> GKIND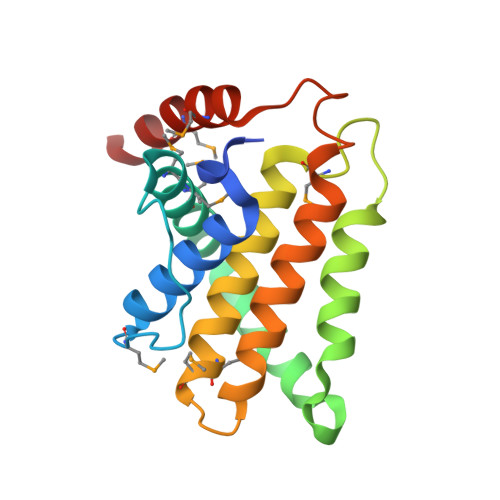WEEPRLDIEGFVVDYFTHRIRQNGMEWFGAPGLPCGVQPEHEMMRVMGTIFEKKHAENFETFCEQLLAVPRISFSPYQDVVRTVGNAQTDQCPMSYGRLIGLISFGGFVAAKMMESVELQGQVRNLFVYTSLFIKTRIRNNWKEHNRSWDDFMTLGKQMKEDYER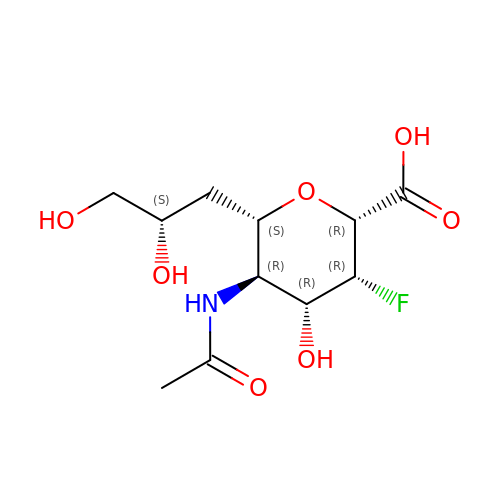5-acetamido-2,6-anhydro-3,5,7-trideoxy-3-fluoro-D-threo-L-galacto-nononic acid | C11 H18 F N O7 | BLSXDTLZOKHJGS-FOVGZEBNSA-N> MTSRKEQLDAFLSRTLSETIAHIPLEKFAQCFPSMKKGKVIAVIHQQLIE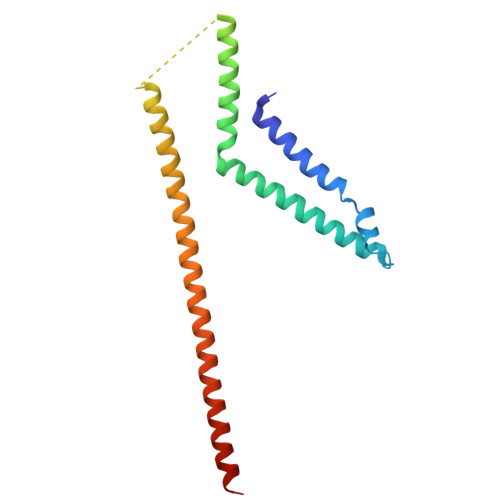FFEKSCKQEYANLIKERDLNKKLDMLDECIHDAEFRKLHGESEVDISNKQPQEILKAHLYSHKRELLDKLNQDLLDIDKENEGLSTQIAAEEKATEDCISRMQSLIQKLEKTVYGMNEKNLAKEA> GGGAEALELLEHCGVCRERLRPEREPRLLPCLHSACSACLGPAAPAAANSSGDGGAAGDGTVVDCPVCKQQCFSKDIVENYFMRDSGSKAATDAQDANQCCTSCEDNAPATSYCVECSEPLCETCVEAHQRVKYTKDHTVRSTGPAKSRDGERTVYCNVHKHEPLVLFCESCDTLTCRDCQLNAHKDHQYQFLEDAVRNQRKLLASLVKRLGDKHATLQKSTKEVRS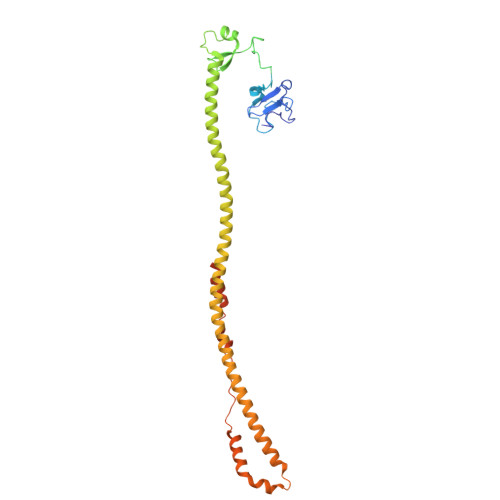SIRQVSDVQKRVQVDVKMAILQIMKELNKRGRVLVNDAQKVTEGQQERLERQHWTMTKIQKHQEHILRFASWALESDNNTALLLSKKLIYFQLHRALKMIVDPVEPHGEMKFQWDLNAWTKSAEAFGKIVAERPGTNSTGPAPMAPPRAPGPLSK> SMAYHQKHGGYGRGGYGR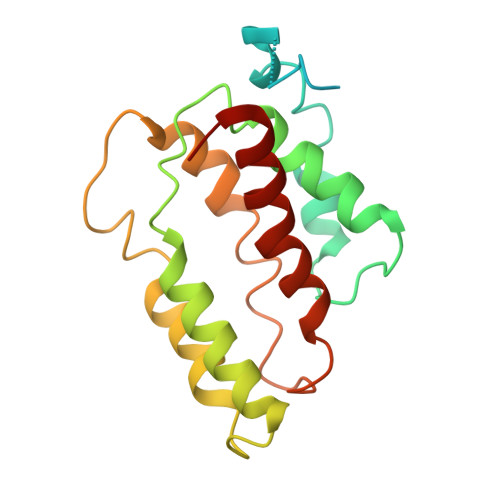QDRPQVDASRLFGESPDVVGIKKMLEGKGKQWEAIQPYFDNVVREAKNFLEWSPNKRLANAVTVAAYLTSQGLKTNQVRKILDMARTTELKVKRGEGDIKDDLVKMRYLLAYTVGKATGQSKYSLDAFHRILDPMLEVLMGSPKKENFEKFYDFLQAVVAYHKFFGGGD>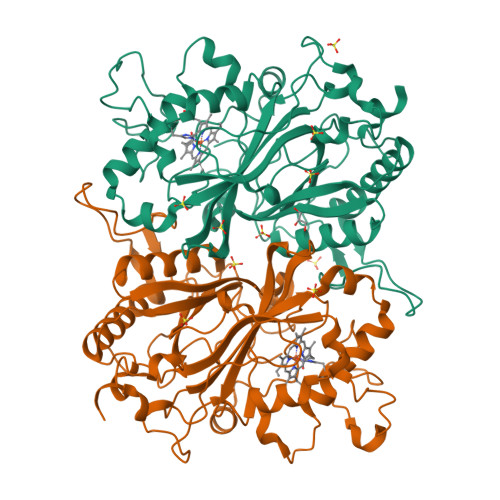[2x]GAMAQKTQSAPGTLSPDARNEKQPFYGEHQAGILTPQQAAMMLVAFDVLASDKADLERLFRLLTQRFAFLTQGGAAPETPNPRLPPLDSGILGGYIAPDNLTITLSVGHSLFDERFGLAPQMPKKLQKMTRFPNDSLDAALCHGDVLLQICANTQDTVIHALRDIIKHTPDLLSVRWKREGFISDHAARSKGKETPINLLGFKDGTANPDSQNDKLMQKVVWVTADQQEPAWTIGGSYQAVRLIQFRVEFWDRTPLKEQQTIFGRDKQTGAPLGMQHEHDVPDYASDPEGKVIALDSHIRLANPRTAESESSLMLRRGYSYSLGVTNSGQLDMGLLFVCYQHDLEKGFLTVQKRLNGEALEEYVKPIGGGYFFALPGVKDANDYFGSALLRV>GSHMEAPILYEDPPEKLTSKDGRAANMKITSWNVDGLRAWVKKNGLDWVRKEDPDILCLQETKCAEKALPADITAMPEYPHKYWAGSEDKEGYSGVAMLCKTEPLNVTYGIGKEEHDKEGRVITAEFPDFFLVTAYVPNASRGLVRLDYRKTWDVDFRAYLCGLDARKPLVLCGDLNVAHQEIDLKNPKGNRKNAGFTPEEREGFTQLLEAGFTDSFRELYPDQAYAYTFWTYMM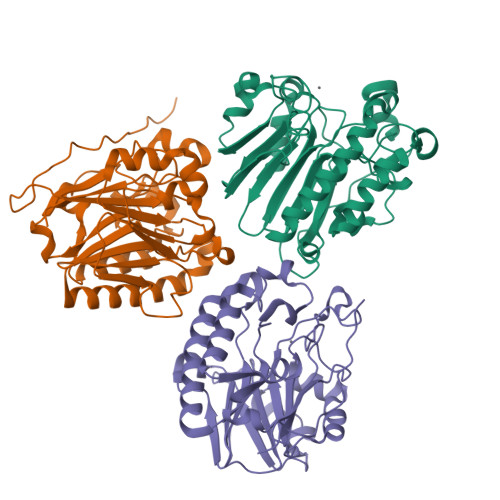NARSKNVGWRLDYFVLSSALLPGLCDSKIRNTAMGSDHCPITLFLAV[3x]> LADHPGELVRTDSPNFLCSVLPTHWRCNKTLPIAFKVVALGDVPDGTLVTVMAGNDENYSAELRNATAAMKNQVARFNDLRFVGRSGRGKSFTLTITVFTNPPQVATYHRAIKITVDGPREPR;> GPIQLWQFLLELLTDKSCQSFISWTGDGWEFKLSDPDEVARRWGKRKNKPKMNYEKLS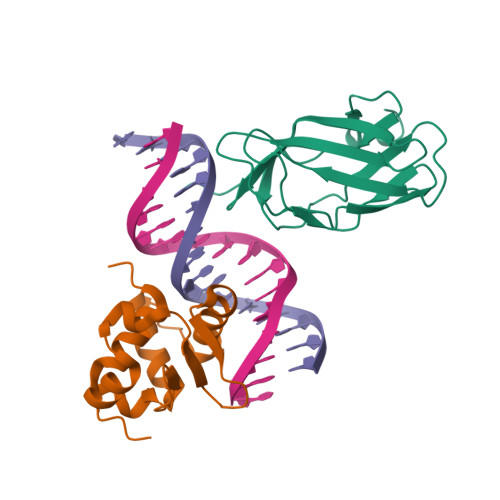RGLRYYYDKNIIHKTAGKRYVYRFVCDLQSLLGYTPEELHAMLDVKPDADE3-(morpholin-4-ylmethyl)-~{N}-[4-(trifluoromethyloxy)phenyl]benzamide | 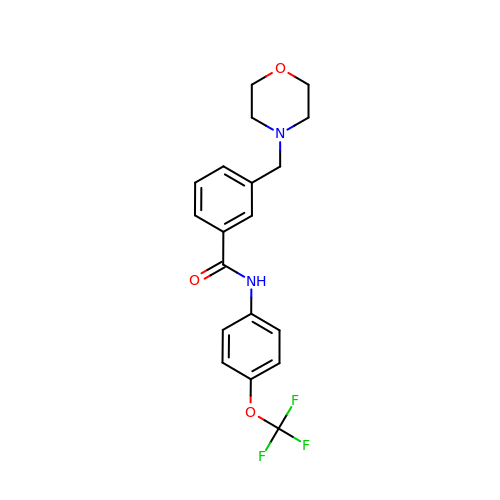C19 H19 F3 N2 O3 | MYWULUKAXYAFSH-UHFFFAOYSA-N4'-O-METHYL-MALTOSYL-ALPHA (1,4)-(Z, 3S,4S,5R,6R)-3,4,5-TRIHYDROXY-6-HYDROXYMETHYL-PIPERIDIN-2-ONE 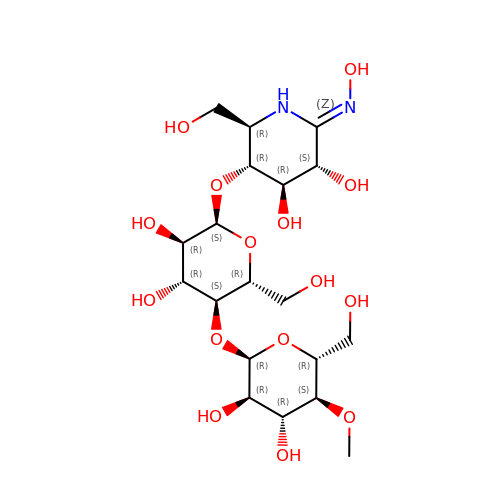| C19 H34 N2 O15 | INFXBQXKGPGIEV-PXPLVWFRSA-N> TASPHALANR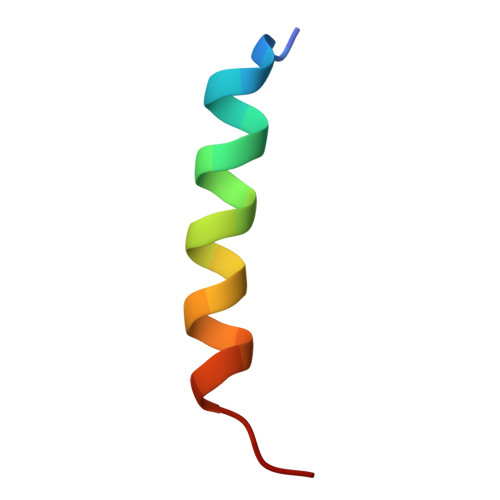LRQLAYRVRSLSS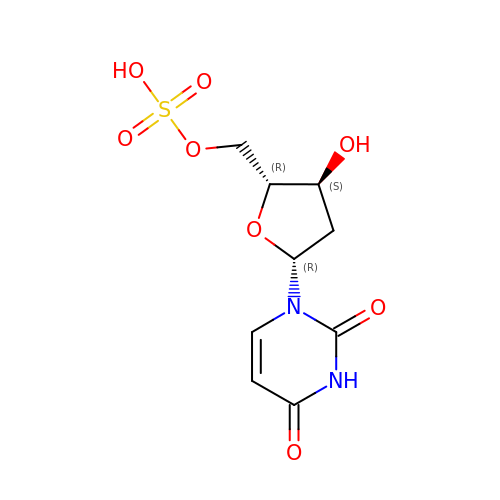2'-deoxy-5'-O-sulfouridine | C9 H12 N2 O8 S | NVGOTALEIZLWEI-SHYZEUOFSA-N>AEEFPVPNGFESAYREVDGVKLHYVKGGQGPLVMLVHGFGQTWYEWHQLMPELAKRFTVIAPDLPGLGQSEPPKTGYSGEQVAVYLHKLARQFSPDRPFDLVAHDIGIWNTYPMVVKNQADIARLVYMEAPIPDARIYRFPAFTAQGESLVWHFSFFAADDRLAETLIAGKERFFLEHFIKSHASNTEVFSERLLDLYARSYAKPHSLNASFEYYRALNESVRQNAELAKTRLQMPTMTLAGGGHGGMGTFQLEQMKAYAEDVEGHVLPGCGHWLPEECAAPM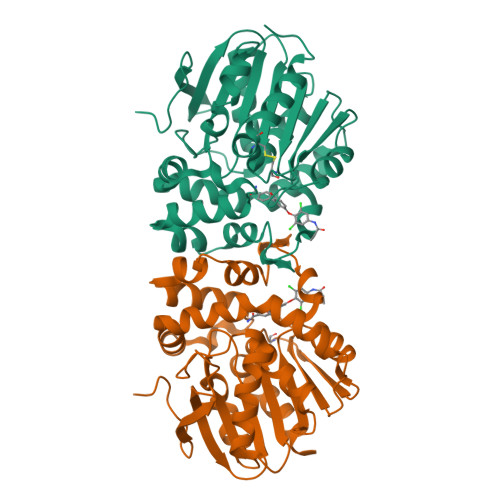NRLVIDFLSRGRHHHHHH[4x]> QGQAAARAAAADLAAGQDDEPRILEAPAPDARRVYVNDPAHFAAVTQQFVIDGEAGRVIGMIDGGFLPNPVVADDGSFIAHASTVFSRIARGERTDYVEVFDPVTLLPTADIELPDAPRFLVGTYPWMTSLTPDGKTLLFYQFSPAPAVGVVDLEGKAFKRMLDVPDCYHIFPTAPDTFFMHCRDGSLAKVAFGTEGTPEITHTEVFHPEDEFLINHPAYSQKAGRLVWPTYTGKIHQIDLSSGDAKFLPAVEALTEA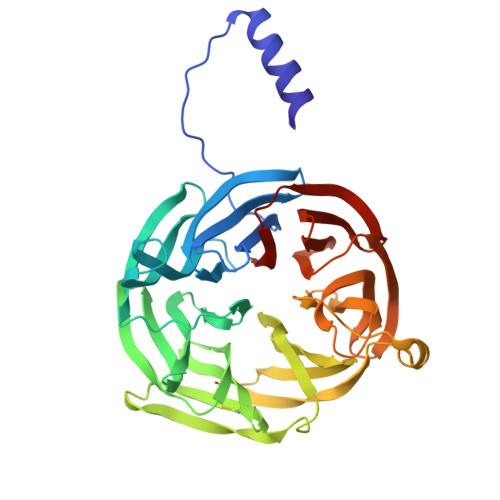ERADGWRPGGWQQVAYHRALDRIYLLVDQRDEWRHKTASRFLVVLDAKTGERLAKFEMGHEIDSINVSQDEKPLLYALSTGDKTLYIHDAESGEELRSVNQLGHGPQVITTADMG>PIELLPETPSQTAGPYVHIGLALEAAGNPTRDQEIWNRLAKPDAPGEHILLLGQVYDGNGHLVRDSFLEVWQADANGEYQDAYNLENAFNSFGRTATTFDAGEWTLHTVKPGVVNNAAGVPMAPHINISLFARGINIHLHTRLYFDDEAQANAKCPVLNLIEQPQRRETLIAKRCEVDGKTAYRFDIRIQGEGETVFFDF[6x];>[6x]PAQDNSRFVIRDRNWHPKALTPDYKTSIARSPRQALVSIPQSISETTGPNFSHLGFGAHDHDLLLNFNNGGLPIGERIIVAGRVVDQYGKPVPNTLVEMWQANAGGRYRHKNDRYLAPLDPNFGGVGRCLTDSDGYYSFRTIKPGPHPWRNGPNDWRPAHIHFGISGPSIATKLITQLYFEGDPLIPMCPIVKSIANPEAVQQLIAKLDMNNANPMDCLAYRFDIVLRGQRKTHFE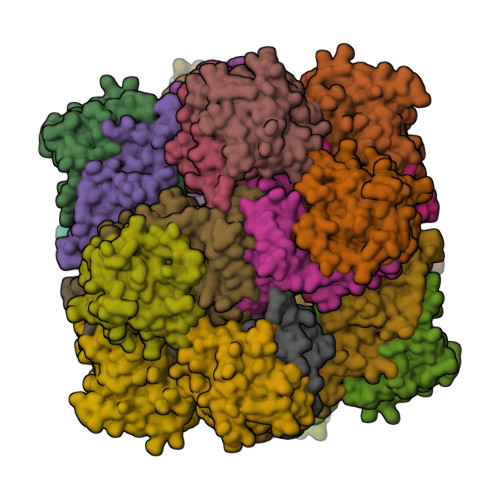NC> GPLGSSQIPASEQETLVRPKPLLLKLLKSVGAQKDTYTMKEVLFYLGQYIMTKRLYDAAQQ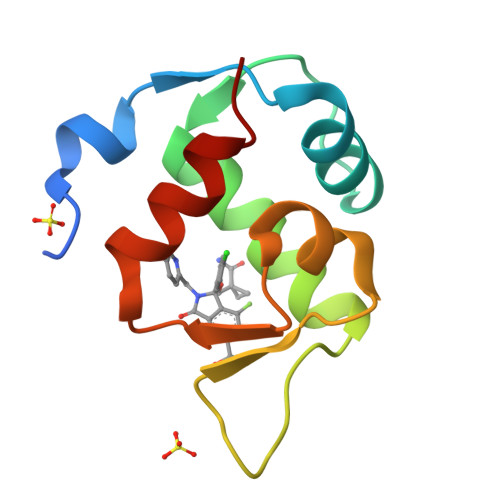HIVYCSNDLLGDLFGVPSFSVKEHRKIYTMIYRNLVV> MAKFFIDRPIFAWVISIFIIAAGIFGIKSLPVSQYPSVAAPTITLHAIYPGASAQVMEGSVLSVIERNMNGVEGLDYMSTSADSSGSGSVSLTFTPDTDENLAQVEVQNKLSEVLSTLPATVQQYGVTVSKARSNFLMIVMLSSDVQSTEEMNDYAQRNVVPELQRIEGVGQVRLFGAQRA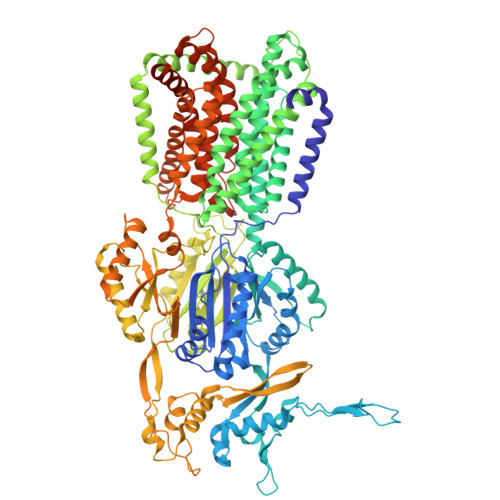MRIWVDPKKLQNYNLSFADVGSALSAQNIQISAGSIGSLPAVRGQTVTATVTAQGQLGTAEEFGNVILRANTDGSNIYLKDVAKVGLGMEDYSSSTRLNGVNTTGMAVMLSNSGNAMATAKAVKERLAVLEKYFPQGMSWKTPYDTSKFVEISIEKVIHTLIEAMVLVFVVMYLFLQNIRYTLIPTIVVPISLLGGFAFISYMGMSINVLTMFAMILVIGIVVDDAIVVVENVERIMAGEGLPPKEATKKAMGQISGAVIGITAVLISVFVPLAMFSGAAGNIYKQFALTMASSIAFSAFLALTLTPALCATMLKTIPKGHHEEKKGFFGWFNKKFDSWTHGYEGRVAKVLRKTFRMMVVYIGLAVVGVFLFMRLPTSFLPTEDQGFVMVSVQLPAGATKERTDATLAQVTQLAKSIPEIENIITVSGFSFSGSGQNMAMGFAILKDWNERTASGSDAVAVAGKLTGMMMGTLKDGFGIAVVPPPILELGNGSGLSINLQDRNNTGHTALLAKRNELIQKMRASGLFDPSTVRAGGLEDSPQLKIDINRAAAAAQGVSFADIRTALASALSSSYVSDFPNQGRLQRVMVQADGDARMQPADILNLTVPNSSGIAVPLSSIATVSWQMGTEQSVRFNGYPAMELSGSPATGVSTGQAMEAVQKMVDELGSGYSLEWGGQSREEAKGGSQTIALYALAAVAVFLVLAALYESWSIPLAVLLVMPLGLAGAAAGVTGRNLFEGLLGSVPSFANDIYFQVGFVTVMGLSAKNAILIIEFAKDLQAQGKSAVEAALEAARLRFRPIIMTSFAFILGVVPLYIAGGASSASQRAIGTTVFWGMLIGTLLSVFLVPLFYVVVRKFFKETAHEHEMAVRHASKAGITGSDDKQY>MKFTEIFPVEDANYPYSAFIASVRKDVIKHCTDHKGIFQPVLPPEKKVPELWLYTELKTRTSSITLAIRMDNLYLVGFRTPGGVWWEFGKDGDTHLLGDNPRWLGFGGRYQDLIGNKGLETVTMGRAEMTRAVNDLAKKKKMLEPQADTKSKLVKLVVMVCEGLRFNTVSRTVDAG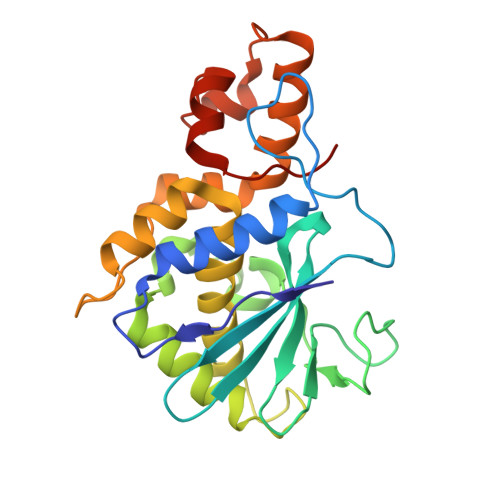FNSQHGVTLTVTQGKQVQKWDRISKAAFEWADHPTAVIPDMQKLGIKDKNEAARIVALVKNQTTAAA[3x]> MEDIIVVALY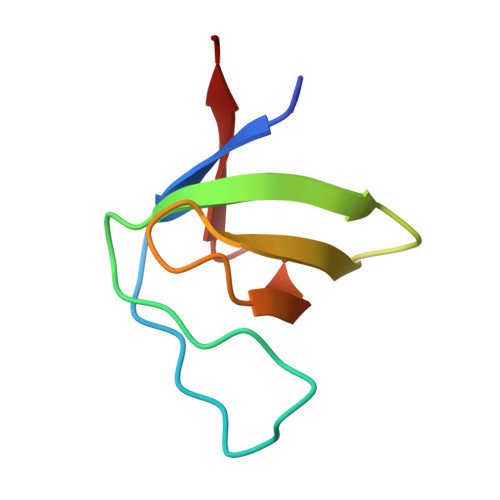DYYSPFSWDLSFQKGDQMVVLEESGEWWKARSLATRKEGYIPSNYVARVDS The 5' region of pre-rRNA that consists of the 5' external transcribed spacer (5' ETS), 18S rRNA and the internal transcribed spacer 1 (ITS1) is co-transcriptionally packed into a terminal ball of ~40 nm in size. These particles represent the earliest assembly intermediates of 40S and are known as the 90S pre-ribosome or the SSU processome. Within 90S, the pre-rRNA is cleaved at sites A0 and A1 in the 5' ETS and site A2 in the ITS1, yielding a 20S pre-rRNA intermediate. The fully assembled 90S contains an unprocessed pre-18S rRNA, U3 snoRNA, approximately 51 assembly factors and 18 r-proteins with a molecular mass of 5.0 megadaltons.

The EM densities were docked with the available crystal structures of yeast 40S ribosome and AFs or homology models of AFs. The 3' major domain RNA is directly bound by Enp1, Emg1, Utp30 and Imp4. Enp1 adopts a superhelix structure and contacts helices 32 and 33. The 3' basal subdomain makes up part of the front face, whereas the 3' beak subdomain sticks out to form the nose. The structural role of helix 44 and six assigned late factors (Utp30, Enp1, Bms1, Rcl1, Pno1, Utp20) in the 90S structure provide insight into the last major assembly event. They function to assemble the 3' major domain (Utp30, Enp1), the 3' minor domain (Pno1) and the 5' basal subdomain (Bms1) and to establish long range connections between ribosomal subdomains (helix 44, Bms1/Rcl1, Utp20).

>GDYKEEEEIVEIDEEDAAMFEQYFKKSDDFNSLSGSYNLADKIMASIREKESQVEDMQDDEPLANEQNTSRGNISSGLKSGEGVALPEKVIKAYTTVGSILKTWTHGKLPKLFKVIPSLRNWQDVIYVTNPEEWSPHVVYEATKLFVSNLTAKESQKFINLILLERFRDNIETSEDHSLNYHIYRAVKKSLYKPSAFFKGFLFPLVETGCNVREATIAGSVLAKVSVPALHSSAALSYLLRLPFSPPTTVFIKILLDKKYALPYQTVDDCVYYFMRFRILDDGSNGEDATRVLPVIWHKAFLTFAQRYKNDITQDQRDFLLETVRQRGHKDIGPEIRRELLAGASREFVDPQEANDDLMIDVN[2x];> GAMSDVSGFSMSSSAIARTETMTVLDDQYDQIINGYENYEEELEEDEEQNYQPFDMSAERSDFESMLDDFLDNYELESGGRKLAKKDKEIERLKEAADEVSKGKLSQRRNRERQEKKKLEKVTNTLSSLKF> MGSSHHHHHHHHSSGLEVLFQGPLGSHMNTRRQQAQNIRNNAAELAANRPHPQHINNKEEYEYRRPKKDGNEPSHIANFTKGLPHDEHTGLLLNSADYDQFVLGIQSGDTTDFARTPLGPAELPKVHGCLSKQKIDCDDDHRSGFWKSQIAQGAAGGDGAKLRAWESAGAGLVFDLEGPDAQAVTMPPAPRLESPELTSEIAEVYSQALLRDIHFSQLRDPGLGDQVNACDSCPTQLSIYEAIDILNTVQIEGQNWFSANCCDLTDDEQARQRPLVTRQNIFRGIAPGDDVGPYLSQFLLIGNNALGGGVFGQEAGHIGYGAIRIDQRVRKATPCKDFMTNFETWLDVQNGADLRGLETYVDADPGKCREFPAYRVITTPRDLATYVHYDALYEAYLNACLILLGMGAPFDPGIPFQKPDVEDKQQGFAHFGGPQILTLVCEAATRGLKAVDFQKFNVHRRLRPEALGGLVDRYKHGKGAGDELKPVAALVEALENVGLLSKVVAHNQLQNQNLDRSGDPSSAGDNYFLPMAFPEGSPMHPSYGAGHATVAGACVTMLKAFFDHGWQLNLGMANGKYISYEPNQDGSSLQQVLLDCPLTVEGELNKIAANISIGRDWAGVHYFTDYIESLRLGEKIAIGILEEQKLTYGENFTMTVPLYDGGSIQI

Vanadium-dependent haloperoxidases (VHPOs) are biotechnologically valuable and operationally versatile biocatalysts. VHPOs are categorized according to the most electronegative halide they can oxidize, leading to chloroperoxidases (VCPOs), bromoperoxidases (VBPOs), and iodoperoxidases (VIPOs). The general mechanism for VHPO-catalyzed reactions is based on the two-electron oxidation of halides. For elucidating the halogen specificity in VHPOs, we chose the vanadium-dependent haloperoxidase AmVHPO from the cyanobacterium Acaryochloris marina MBIC 1101721.

In contrast, in R425S, this section consolidated in a loop structure, strongly influenced by the introduced serine residue (highlighted in blue). The hypothesis that this loop is responsible for the halogen specificity is supported by the crystal structure analyses of the AmVHPO mutant R425D, which has no chlorination activity and lacks a structured conformation of residues 400–405. In the R425D mutant, this motif is only partially present (residue 390–400), so no interactions with 7 can occur. These molecular findings agree with the wild-type structure, in which residues 390–404 are also flexible. At the same time, no activity was measured in the presence of the wild-type enzyme or the R425D mutant. No co-crystal structure of 7 and the R425D or the wild-type enzyme could be obtained. An isosteric phosphate, obtained from the reservoir solution, replaced the cofactor vanadate in the enzyme crystals. Both mutant structures feature the identical characteristic assembly of a hexamer of dimers, arranged in a “head-to-tail” orientation with superimposable key catalytic residues when compared to the wild-type.Here, we present the discovery of a promiscuous allosteric site in SMYD2, a unique member of the protein lysine methyltransferase family characterized by the co-presence of the SET and MYND domains. SMYD2 is a critical regulator of numerous cellular processes, methylating both histone and non-histone proteins to control chromatin remodeling, DNA damage response, cell cycle progression, cell differentiation, cell survival, and inflammation. We have determined four crystal structures of SMYD2, including a wild-type protein structure in complex with a PARP1 peptide, a wild-type protein structure in complex with an ethylene glycol polymer (PEG), and two structures of SMYD2 mutants. In all structures, SMYD2 maintains a bilobal fold, with the N- and C-lobes displaying a similar orientation and a similar degree of opening.

L351A/W356A is a secondary-binding-site mutation that targets both subsites M and L, while F184A targets the target lysine access channel at the active site. The F184A mutant was also crystallized with the PARP1 peptide, but no peptide is found in either the substrate binding site or the secondary binding site, suggesting that this mutation also disrupts binding at both sites. Phe184, together with the two other aromatic residues Tyr240 and Tyr258, forms the target lysine access channel. Mutating Phe184 to the smaller alanine (F184A) widens this channel significantly. In the wild-type structure, the target lysine fits snugly within the channel. The mutation likely disrupts this precise fit, leading to the loss of binding. Despite no peptide being identified, the secondary binding site contains PEG-like electron densities. The results showed that the peptide binds in a 2:1 ratio with the wild-type protein, which changes to 1:1 with the F184A mutation. In contrast, the F184A mutation at the target lysine access channel abolishes the methyltransferase activity of SMYD2 on all tested substrates, even though these substrates, except for the PARP1 peptide, can still bind to the mutant.

> MRAEGLGGLERFCSPGKGRGLRALQPFQVGDLLFSCPAYAYVLTVNERGNHCEYCFTRKEGLSKCGRCKQAFYCNVECQKEDWPMHKLECSPMVVFGENWNPSETVRLTARILAKQKIHPERTPSEKLLAVKEFESHLDKLDNEKKDLIQSDIAALHHFYSKHLGFPDNDSLVVLFAQVNCNGATIEDEELSHLGSAIFPDVALMNHSCCPNVIVTYKGTLAEVRAVQEIKPGEEVFTSYIDLLYPTEDRNDRLRDSYFFTCECQECTTKDKDKAKVEIRKLSDPPKAEAIRDMVRYARNVIEEFRRAKHYKSPSELLEICELSQEKMSSVFEDSNVYMLHMMYQAMGVCLYMQDWEGALQYGQKIIKPYSKHYPLYSLNVASMWLKLGRLYMGLEHKAAGEKALKKAIAIMEVAHGKDHPYISEIKQEIESH>DQSFLW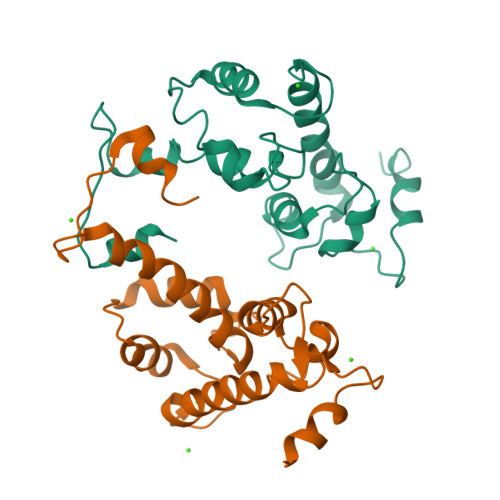NVFQRVDKDRSGVISDTELQQALSNGTWTPFNPVTVRSIISMFDRENKAGVNFSEFTGVWKYITDWQNVFRTYDRDNSGMIDKNELKQALSGFGYRLSDQFHDILIRKFDRQGRGQIAFDDFIQGCIVLQRLTDIFRRYDTDQDGWIQVSYEQYLSMVFSIV[8x]> ESC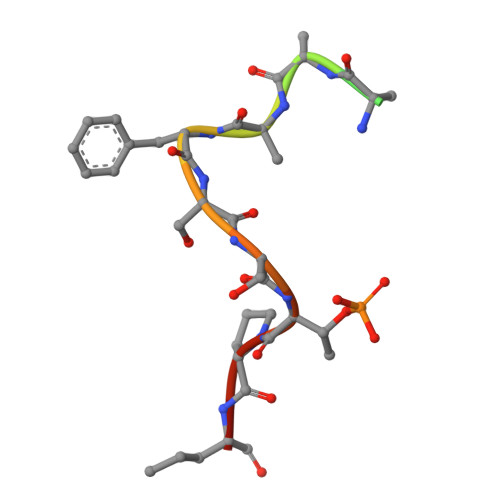FTNAAFSSTPKK> MQRNTYNKVGLYILSLAMLFVFIIILTAKIPFCFTSDCSFIGLKKLVLTNIVPIVCFVFFLFSIYFYNRLKNITKYNGQDSVKITSCQSESYESLTFLATYIVPFMGFSFEDMQKNIAYLLLVVVIGIIFIKTDKYYANPTLALFGFKLYRVNILHPGSGETKNLIAISNDVLKVDDNVYYSFFDEFVFIARKKIDYKDDDDK;>MTTQQLKEKISKIIDNFSGIRVVFTTTANELKLSRIEGSALNSIAEGFIDKIKEDIINNEDLTSPLLSNFDDRKNALFKFDYEQYPEEFNKITQAIAIPPNSQDYYNPLNKFTDVKGIIILISGDNKCLALYKNKTNLAVLRNSRKMFNLVPDPDGYLKQLPNEILRLDFNYDLFSIGEDFYIKNHKTLETQMKFHQVIEAQAVIALNSLRDSLLIEDISGLEKSSREISFARKLAKISKHSPVLGKIDTKTIIDYVSQHKY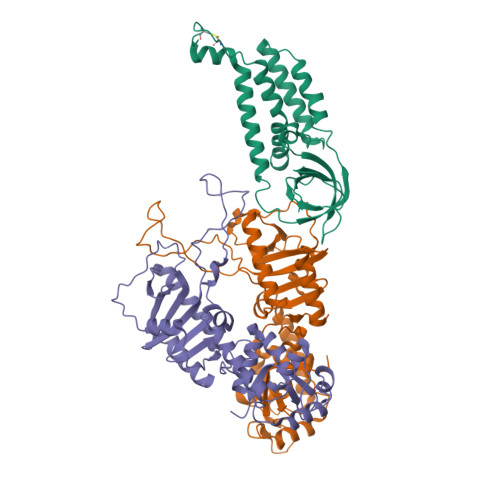LSAILQINEAGDKLLIKTKTSQKHFIKLMSDDYLQSDLTKIIYMSIAKDRLDEHHHHHH[2x]>ASMTGGQQMG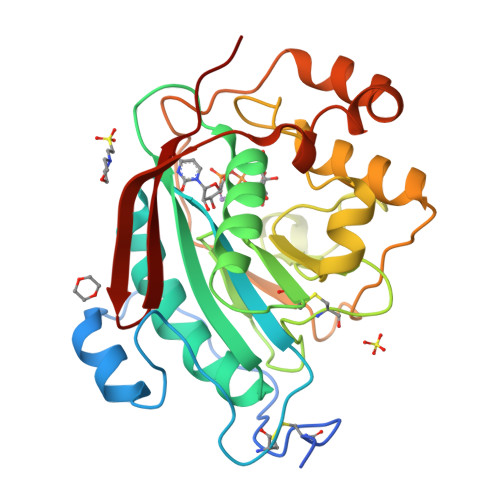RGSSLTACPEESPLLVGPMLIEFNIPVDLKLVEQQNPKVKLGGRYTPMDCISPHKVAIIIPFRNRQEHLKYWLYYLHPILQRQQLDYGIYVINQAGESMFNRAKLLNVGFKEALKDYDYNCFVFSDVDLIPMNDHNTYRCFSQPRHISVAMDKFGFSLPYVQYFGGVSALSKQQFLSINGFPNNYWGWGGEDDDIYNRLAFRGMSVSRPNAVIGKTRMIRHSRDKKNEPNPQRFDRIAHTKETMLSDGLNSLTYMVLEVQRYPLYTKITVDIGTPS[2x]> MEQETLEQVHLTEDGGVVKTILRKGEGGEENAPKKGNEVTVHYVGKLESSGKVFDSSRERNVP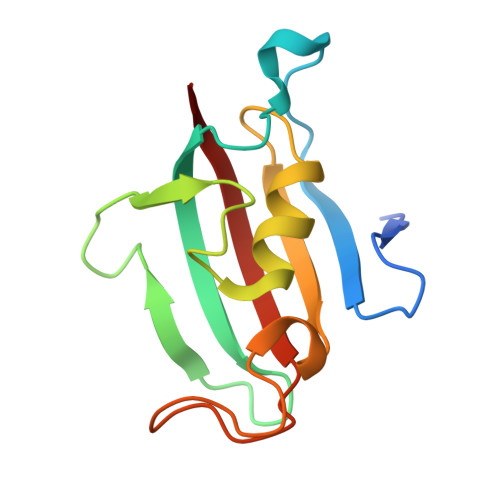FKFHLGQGEVIKGWDICVASMTKNEKCSVRLDSKYGYGEEGCGESIPGNSVLIFEIELISFRE> AVKLSHVEKDFIAFYSTTPHHLSYRDKTGGSYFITRLISCFRKH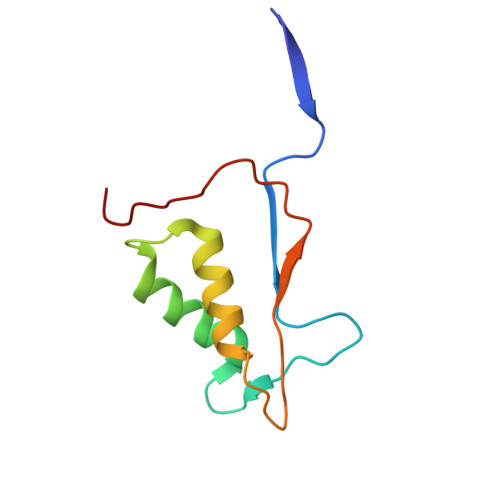ACSCHLFDIFLKVQQSFEKASIHSQMPTIDRATLTRYFYLFPGN>SMAALAPLPPLPAQFKSIQHHLRTAQEHDKRDPVVAYYCRLYAMQTGMKIDSKTPECRKFLSKLMDQLEALKKQLGDNEAITQEIVGCAHLENYALKMFLYADNEDRAGRFHKNMIKSFYTASLLIDVITVFGELTDENVKHRKYARWKATYIHNCLKNGETP[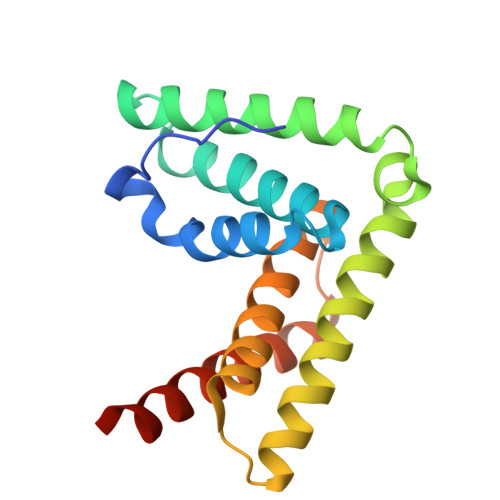3x]>GSMASAPLRVYVQCNPLLDVSAHVSDEFLVKYGLERGTAILLSERQKGIFDDIEKMPNVRYVPGGSGLNVARVAQWMQQAYKGKFVTYVGCIADDRYGKVLKEAAEHEGIVMAVEHTTKAGSGACAVCITGKERTLVADLGAANHLSSEHMRSPAVVRAMDESRIFYFSGFTLTVDVNHVLQACRKAREVDGLFMINLSAPFIMQFFSAQLGEVLPYTDIIVANRHEAKEFANMMKWDTDCVEEIARRAVSEVPYTGTKGRVVVFTRDIESTVLATKDGVETVPVPQLDQDKVIDMNGAGDAFMGGFLSAYAVGKDLRRCCETGHYTAQEVIQRDGCSFPEKPSFSP[2x]

Adenosine kinase (EC 2.7.1.20, ATP:adenosine 5′-phosphotransferase) catalyzes the phosphorylation of adenosine to adenosine monophosphate (AMP) in presence of Mg2+ and utilizing ATP as the preferred phosphoryl donor. Recently T. brucei adenosine kinase (TbAK) was identified as a key enzyme mediating high affinity adenosine salvage in the purine salvage pathway. The overall structures of both TbrAK in complex with AP5A and compound 1 contain a mixed fold and consist of 12 α-helices and 14 β-strands that form two distinct domains. A common property of adenosine kinases from various organisms is their control via substrate-inhibition to prevent non-physiologically high intracellular purine nucleotide levels, and recently it has been shown that TbrAK activity is strongly inhibited by its substrate adenosine.

The two molecules (A and B) found in the asymmetric unit were not related by proper non-crystallographic symmetry and exhibited a mixed hydrophilic/hydrophobic contact interface typical for crystal contacts. Apparently, the molecules do not form a functional dimer and thus could be considered as two separate monomers. The bisubstrate inhibitor AP5A was co-crystallized with TbrAK which adopts the closed conformation in presence of this compound. The electron density of AP5A was clearly resolved in the structure and provides a detailed view into the adenosine and the ATP binding site. AP5A exhibits an extensive hydrogen bonding pattern with the protein either through direct or water-mediated interactions. The interactions in the adenosine binding pocket are mainly water-mediated, apart from the side chain NH2 group of N13 which makes a hydrogen bond with nitrogen N1 of adenosine and the side chain of D17 which forms bidentate interactions with the two OH-groups of the ribose. The phosphate groups of AP5A are stabilized by water mediated interactions and by the side chain NH2 groups of R132 and N222 and the backbone nitrogen of A297. The adenosine part of AP5A in the ATP-binding pocket shows hydrogen bonds to the side chains of Q288 (to the free NH2 group of adenine) and Q327 (to a nitrogen atom of the pyrimidine ring of adenine), and the ribose moiety is stabilized by backbone interactions with D266 and T270.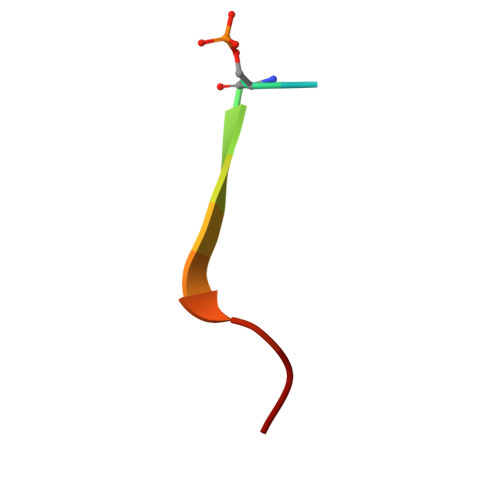> SDDSDIVTLEPPK The stringent response enables bacteria to respond to nutrient limitation and other stress conditions through production of the nucleotide-based second messengers ppGpp and pppGpp, collectively known as (p)ppGpp. Here, we report that (p)ppGpp inhibits the signal recognition particle (SRP)-dependent protein targeting pathway, which is essential for membrane protein biogenesis and protein secretion. More specifically, (p)ppGpp binds to the SRP GTPases Ffh and FtsY, and inhibits the formation of the SRP receptor-targeting complex, which is central for the coordinated binding of the translating ribosome to the SecYEG translocon. Briefly, SRP recognizes hydrophobic signal sequences in the context of translating ribosomes, and SRP bound to ribosome-nascent chain complexes (RNCs) in turn interacts in a GTP-dependent manner with its receptor FtsY, also a GTPase, which localizes at the cytoplasmic membrane periphery of bacteria via a membrane-targeting sequence.

Determination of the dissociation constants (KD) of (Ec)Ffh-NG revealed an affinity of 7.9 ± 1.9 µM for ppGpp-binding while its counterpart GDP exhibited an affinity of 2.2 ± 0.6 µM. For the NG domain of the SRP-receptor (Ec)FtsY a KD of 21.7 ± 5.4 µM for ppGpp and 9.8 ± 1.1 µM for GDP were obtained. These KD values show that ppGpp exhibits similar binding affinities as its GDP counterpart for the SRP-GTPases Ffh and FtsY. We determined the crystal structures of the pppGpp-bound NG domains of (Ec)Ffh and (Ec)FtsY at resolutions of 2.5 and 2.4 Å, respectively, as well as the crystal structures of (Bs)Ffh and (Ec)Ffh in complex with ppGpp and Mg2+ at resolutions of 2.5 and 2.8 Å, respectively. The ppGpp or pppGpp molecules are bound to the G domains of Ffh and FtsY and occupy the canonical guanosine nucleotide-binding site. In detail, the guanine moiety of (p)ppGpp is recognized by the well-described aspartate of the G4 element responsible for the discrimination of guanosine nucleotides by P-loop type GTPases. The α-, β-, and γ-phosphates of (p)ppGpp are coordinated by the G1-element (P-loop), and by residues originating from the switch I and II regions including the G2 and G3 elements, respectively. The δ- and ε-phosphate, which are covalently bound to the 3′-OH group of the ribose moiety and discriminate (p)ppGpp from its GDP/GTP counterparts, point away from the active sites of both GTPases. Both phosphates are not coordinated or form any obvious contacts to the GTPases of Ffh and FtsY. The missing coordination leads to a high flexibility of the δ- and ε-phosphate, as observed in the crystals of (Ec)Ffh with pppGpp. We conclude that ppGpp and pppGpp interact with the SRP-GTPases Ffh and FtsY in the same way as its counterparts GDP and GTP, respectively, also providing the structural explanation for their comparable KD values (see above).

> MGFDNLTDRLSRTLRNISGRGRLTEDNVKDTLREVRMALLEADVALPVVREFINRVKEKAVGHEVNKSLTPGQEFVKIVRNELVAAMGEENQTLNLAAQPPAVVLMAGLQGAGKTTSVGKLGKFLREKHKKKVLVVSADVYRPAAIKQLETLAEQVGVDFFPSDVGQKPVDIVNAALKEAKLKFYDVLLVDTAGRLHVDEAMMDEIKQVHASINPVETLFVVDAMTGQDAANTAKAFNEALPLTGVVLTKVDGDARGGAALSIRHITGKPIKFLGVGEKTEALEPFHPDRIASRILGMGDHHHHHH> MAHHHHHHGPNTNPVAAWKALKEGNERFVAGRPQHPSQSVDHRAGLAAGQKPTAVIFGCADSRVAAEIIFDQG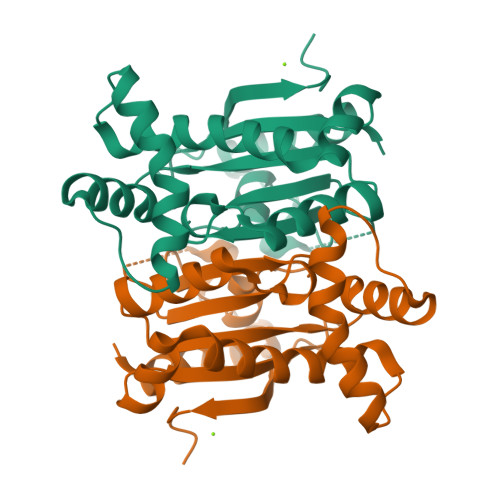LGDMFVVRTAGHVIDSAVLGSIEYAVTVLNVPLIVVLGHDSCGAVNAALAAINDGTLPGGYVRDVVERVAPSVLLGRRDGLSRVDEFEQRHVHETVAILMARSSAISERIAGGSLAIVGVTYQLDDGRAVLRDHIGNIGEEV>MVLDVTKDHWLLYVLLAQLPVMVLFRKDNDEEAKKVEYIVRELAQEFDGLIMVFELDTNKAPEIAKKYNITTTPTVAFFKNGEDKSVLIGAIPKDQL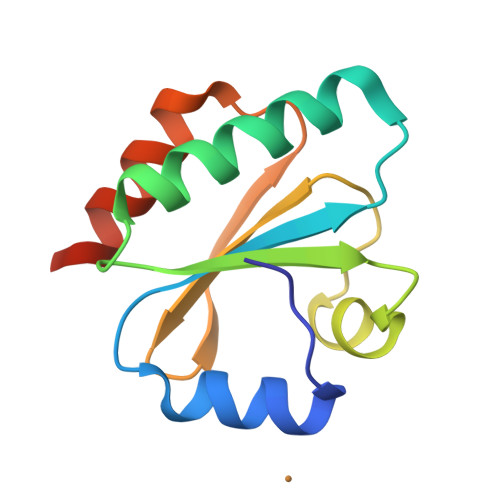RDEILKYLGHHHHHH[8x]>MKEIKLILTDIDGVWTDGG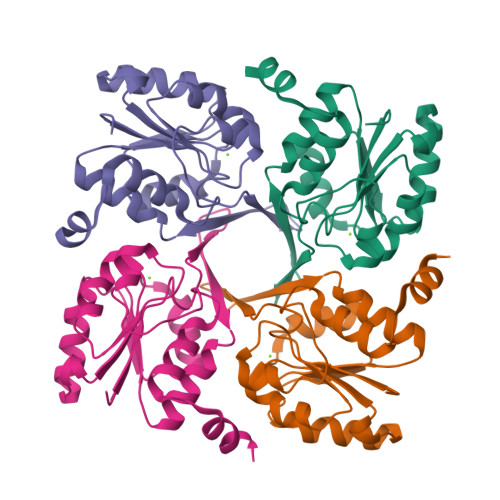MFYDQTGNEWKKFNTSDSAGIFWAHNKGIPVGILTGAKTEIVRRRAEALKVDYLFQGVVDKLSAAEELCNELGINLEQVAYIGDDLNDAKLLKRVGIAGVPASAPFYIRRLSTIFLEKRGGEGVFREFVEKVLGINLEDFIAVIQ[8x]>DPFTMFEEINDFETAFKRLLNEVLEFDLQNPLKDVKKVLCIEPHPDDCVIGMGGTIKRLTDRGIEVIYICMTDGYMGTTDENITGHELAQIRRKEEEESAKMLGVKKIYWLNYRDTELPYSREVRKDLVKIIRKEKPDGVFLPDPWLPYEAHPDHRATGFLALDAVAFSPLPNFSNIDLDIGLKPHSVSFIGLYYTSRPNYFVDITDVMDLKLKAIRAHKSQFPDDIWETWEPFLRTVALYYGQKAGVKYAEGFRIMPGLFYHITPFAELI[12x]

Deacetylase from the extremophile Pyrococcus chitonophagus has been analyzed by X-ray crystallography, small-angle X-ray scattering, differential scanning calorimetry, isothermal titration calorimetry and NMR to determine its structure, thermodynamics and enzymatic properties. It is a hexameric, zinc-containing metalloenzyme that retains its structural integrity up to temperatures slightly exceeding 100 °C. It removes the acetyl group specifically from the non-reducing end of the sugar substrate. Pch-Dac crystallizes as ‘a dimer of trimers’, with two doughnut-shaped trimers stacked back-to-back along a molecular three-fold axis, with a 8–10 Å channel through the middle of this assembly.

Three crystal forms were analyzed, including monoclinic crystals of the protein-substrate complex (Pch-Dac-lig), having two protein hexamers in the crystal’s asymmetric unit and trigonal crystals of the unliganded protein (Pch-Dac), having half a hexamer in the asymmetric unit, with the other half being related by the crystallographic two-fold axis. A (GlcNAc)2 substrate molecule was found in each substrate-binding cavity of the 12 crystallographically independent subunits in the Pch-Dac-lig structure. The electron density clearly indicated two connected sugar rings. The GlcNAc moiety that is closer to the active site is held in place by a network of hydrogen bonds to the surrounding protein residues. The N-acetyl group is directed toward Zn2+ and its carbonyl oxygen atom completes the tetrahedral coordination sphere of the Zn2+ ion (the Zn2+ to O distance is 2.1 ± 0.03 Å). The substrate’s N-acetyl group is flanked by Asp42 and His259* (* denotes that the residue comes from the neighboring subunit). Its position is equidistant from the two flanking residues (3.5 ± 0.2 Å from the carbonyl oxygen to Nε2 of His259 and to Oδ1 of Asp42). The methyl part of the N-acetyl group of the substrate is lodged in a hydrophobic pocket formed by Ile46, Phe219, Trp227 and Ile260*. The substrate approaches the Zn2+ ion in a monodentate manner, displacing the water molecule with the oxygen atom of its acetyl group. There is no evidence in the electron density of a water molecule that could act as the hydrolytic water and there is no place where a water molecule could be fitted in the immediate vicinity of the active site.Here structural analysis of hydroxyketoacid aldolase from Sphingomonas wittichii RW1 (SwHKA) revealed a dynamic movement of the metal cofactor between two coordination spheres without protein scaffold rearrangements. Holo‐SwHKA forms a trimer of homodimers, in which each monomer adopts an (α/β)8 triosephosphate isomerase (TIM) barrel fold. In total, holo‐SwHKA contains six equivalent active sites; each of which is formed from amino acids from two different domain‐swapped dimers. The transition from M2+ R to M2+ A,S is induced by bidentate substrate binding and occurs without a concomitant rearrangement of the protein scaffold.

In the presence of ketoacids, bidentate substrate coordination affords M2+ A,S as the lowest energy complex and predominant state in crystal structures. The M2+ A,S complex is additionally stabilized by side chain interactions from the protein environment with the coordinated substrate. With d‐glyceraldehyde (DGA) and HPA in the active site the position that phosphate occupied is fully taken. The DGA is in a similar position as phosphate, interacting through hydrogen bonds with R69 and R120′ from the adjacent monomer. These interactions, and in particular the hydrogen bond to R69, orient the aldehyde for the nucleophilic attack by HPA. In SwHKA the equivalent loop (residues 117′–121′) is shown to tightly interact with the aldehyde molecule through R120′. Whether these interactions are associated with SwHKA stereoselectivity for the (3S,4S)‐isomer is unclear.

> MHHHHHHNKVRTCWNEGRPALAGWLQLPGTLHAEALARLDYDAVVIDMQHSPIDFGQVAPMLIAIELGGAEPFVRTQVNDPSDIMKLLDAGAYGIIAPMVNTRAEAQTLASALHYSPRGLRSFGPRRPSLRYGSGYLAQASETVVGLAMIETREALANIDEILSVDGIDGVFIGPTDLALDLGHAPLVDTEEAEVVSAIAHVRERAHAAGKRVGIFCGSGGFARVKLAEGFDFVTAAPDLAMLSAAARQVIADARAL(3~{S},6~{S})-3-[(2,6-dimethyl-4-oxidanyl-phenyl)methyl]-6-[(4-hydroxyphenyl)methyl]piperazine-2,5-dione | C20 H22 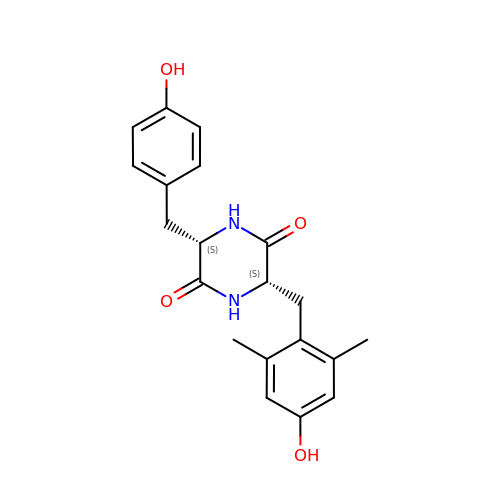N2 O4 | QLYLWUHZTOECNX-ROUUACIJSA-N> MIMDKENTFSYKQAITGTAVSTNVIDLGVSRDIGKGVPVPIIIQVVE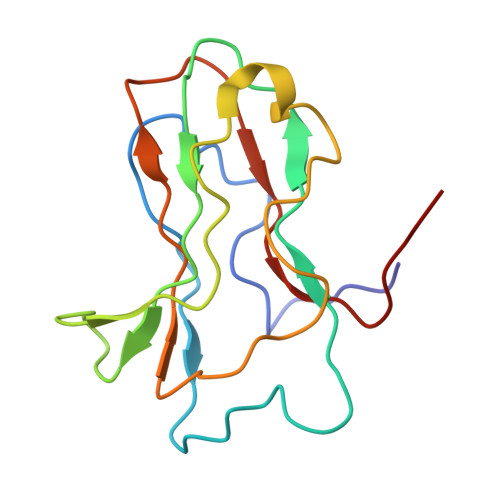DFADATSLTATLQTSETENFSSATTLATSGAVPVADLTAGKQLAVQYMPLGTQRYLRVNYTVSGTATAGAVTAGVVMSHQQND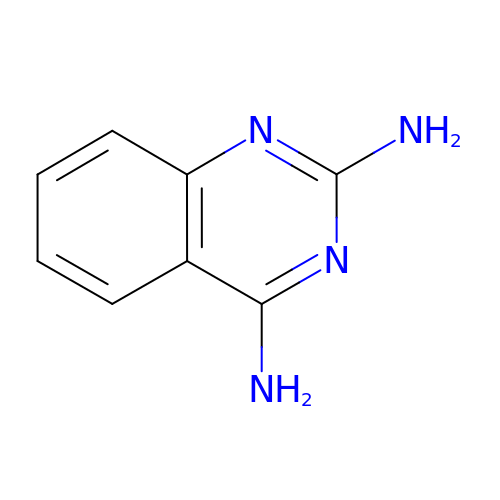quinazoline-2,4-diamine | C8 H8 N4 | XELRMPRLCPFTBH-UHFFFAOYSA-N> HGMSQPACTARRRTRVLILGVNGFIGNHLTERLLREDHYEVYGLDIGSDAISRFLNHPHFHFVEGDISIHSEWIEYHVKKCDVVLPLVAIATPIEYTRNPLRVFELDFEENLRIIRYCVKYRKRIIFPSTSEVYGMCSDKYFDEDHSNLIVGPVNKPRWIYSVSKQLLDRVIWAYGEKEGL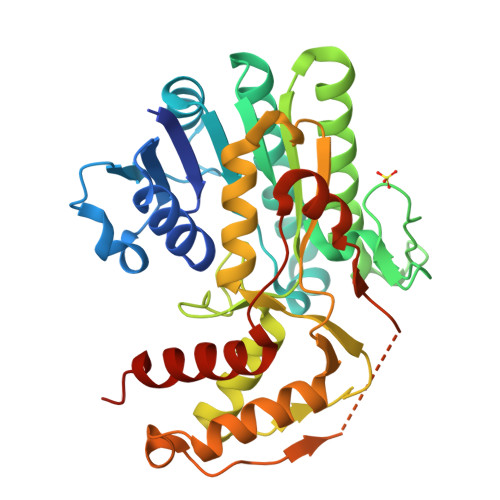QFTLFRPFNWMGPRLDNLNAARIGSSRAITQLILNLVEGSPIKLIDGGKQKRCFTDIRDGIEALYRIIENAGNRCDGEIINIGNPENEASIEELGEMLLASFEKHPLRHHFPPFAGFRVVESSSYYGKGYQDVEHYKPSIRNAHRCLDWEPKIDMQETIDETLDFFLRTVDLTDKPS> LQDLVRGIRNHKEDEAKYISQCIDEIKQELKQDNIAVKANAVCKLTYLQMLGYDISWAAFNIIEVMSASKFTFKRIGYLAASQSFHEGTDVIMLTTNQIRKDLSSPSQYDTGVALTGLSCFVTPDLARDLANDIMTLMSHTKPYIRKKAVLIMYKVFLKYPESLRPAFPRLKEKLEDPDPGVQSAAVNVICELARRNPKNYLSLAPLFFKLMTSSTNNWVLIKIIKLFGALTPLEPRLGKKLIEPLTNLIHSTSAMSLLYECVNTVIAVL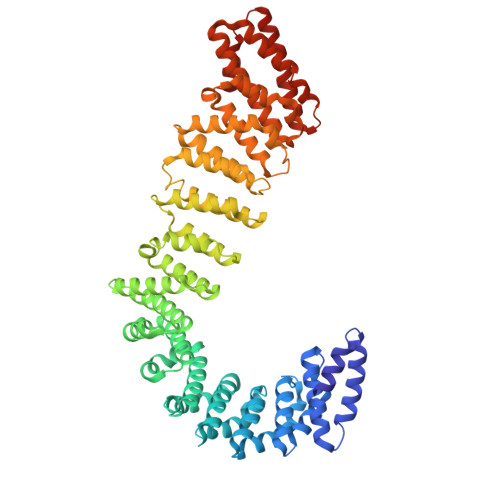ISLSSGMPNHSASIQLCVQKLRILIEDSDQNLKYLGLLAMSKILKTHPKSVQSHKDLILQCLDDKDESIRLRALDLLYGMVSKKNLMEIVKKLMTHVDKAEGTTYRDELLTKIIDICSQSNYQYITNFEWYISILVELTRLEGTRHGHLIAAQMLDVAIRVKAIRKFAVSQMSALLDSAHLLASSTQRNGICEVLYAAAWICGEFSEHLQEPHHTLEAMLRPRVTTLPGHIQAVYVQNVVKLYASILQQKEQAGEAEGAQAVTQLMVDRLPQFVQSADLEVQERASCILQLVKHIQKLQAKDVPVAEEVSALFAGELN>AETTPWGQTFVGATVLSDSQAGNRTICIIDSGYDRSHNDLNANNVTGTNNSGTGNWYQPGNNNAHGTHVAGTIAAIANNEGVVGVMPNQNANIHIVKVFNEAGWGYSSSLVAAIDTCVNSGGANVVTMSLGGSGSTTTERNALNTHYNNGVLLIAAAGNAGDSSYSYPASYDSVMSVAAVDSNLDHAAFSQYTDQVEISGPGEAILSTVTVGEGRLADITIGGQSYFSNGVVPHNRLTPSGTSYAPAPINASATGALAECTVNGTSFSCGNMANKICLVERVGNQGSSYPEINSTKACKTAGAKGIIVYSNSAL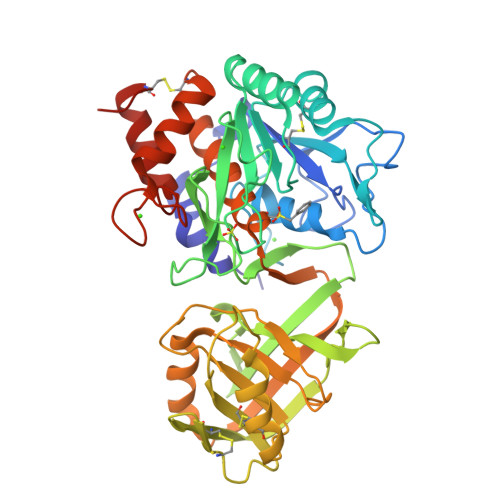PGLQNPFLVDANSDITVPSVSVDRATGLALKAKLGQSTTVSNQGNQDYEYYNGTSMATPHVSGVATLVWSYHPECSASQVRAALNATADDLSVAGRDNQTGYGMINAVAAKAYLDESCTGPTDPGTG[2x]> GSPGISGGGGGILDSMAS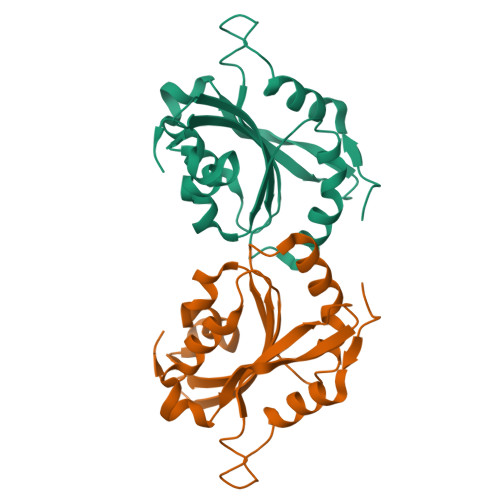GVAVSDGVIKVFNDMKVRKSSTPEEVKKRKKAVLFCLSEDKKNIILEEGKEILVGDVGQTVDDPYATFVKMLPDKDCRYALYDATYETKESKKEDLVFIFWAPESAPLKSKMIYASSKDAIKKKLTGIKHELQANCYEEVKDRATLAEKLGGSAVISLEGKPL> LVATTSSKIYDNKNQLIADLG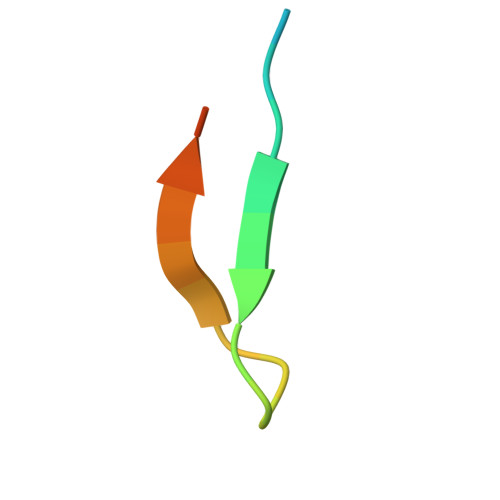SER>SRKTYTLTDYLKNTYRLKLYSLRWISDHEYLYKQENNILVFNAEYGNSSVFLENSTFDEFGHSINDYSISPDGQFILLEYNYVKQWRHSYTASYDIYDLNKRQLITEERIPNNTQWVTWSPVGHKLAYVWNNDIYVKIEPNLPSYRITWTGKEDIIYNGITDWVYEEEVFSAYSALWWSPNGTFLAYAQFNDTEVPLIEYSFYSDESLQYPKTVRVPYPKAGAVNPTVKFFVVNTDSLSSVTNATSIQITAPASMLIGDHYLCDVTWATQERISLQWLRRIQNYSVMDICDYDESSGRWNCLVARQHIEMSTTGWVGRFRPSEPHFTLDGNSFYKIISNEEGYRHICYFQIDKKDCTFITKGTWEVIGIEALTSDYLYYISNEYKGMPGGRNLYKIQLSDYTKVTCLSCELNPERCQYYSVSFSKEAKYYQLRCSGPGLPLYTLHSSVNDKGLRVLEDNSALDKMLQNVQMPSKKLDFIILNETKFWYQMILPPHFDKSKKYPLLLDVYAGPCSQKADTVFRLNWATYLASTENIIVASFDGRGSGYQGDKIMHAINRRLGTFEVEDQIEAARQFSKMGFVDNKRIAIWGWSYGGYVTSMVLGSGSGVFKCGIAVAPVSRWEYYDSVYTERYMGLPTPEDNLDHYRNSTVMSRAENFKQVEYLLIHGTADDNVHFQQSAQISKALVDVG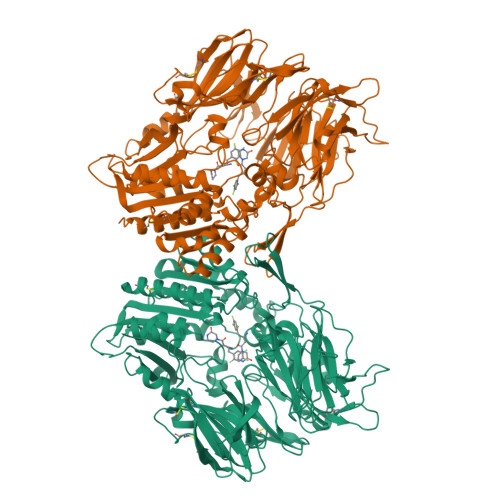VDFQAMWYTDEDHGIASSTAHQHIYTHMSHFIKQCFSLP[2x]> MNTNNIKKYAPQARNQFRDAVIQKLTTLGISADKKGNLQIADAELVGETMRYGQFDYPKSTLTRRDRLVKRAREQGFDVLVEHCAYTWFNRLCAIRYMEIHGYLDHGFHMLSHPDNPTGFEVLDHVPEVAEALLPEKKAQLVEMKLSGNQDEAIYRELLLAQCHALHRAMPFLFEAVDDEAELLLPDNLTRTDSILRGLVDGIPEEDWQEVEVIGWLYQFYISEKKDAVIGKVVKSEDIPAATQLFTPNWIVQYLVQNSVGRQWLQTYPDSPLKGKMDYYIEPAEQTPEVQAQLAAITPASIEPESIKVLDPACGSGHILIEVYNVLKNIYEERGYRARDIPQLILENNIFGLDIDDRAAQLSGFALLMMARQDDRRIFTRDVRLNIVSLQESLHLDIAKLWQQLNFHQQNQTGSMGDMFAENTALAHTDSAEYQLLMRTLKRFVNAKTLGSLIQVPQEEEAELKAFLEALYRMEQ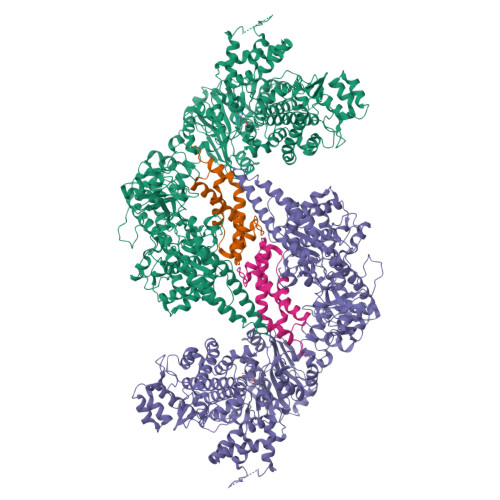EGDFQQKAAAKAFIPYIQQAWILAQRYDAVVANPPYMGGKGMNSELKEFAKNNFPDSKADLFAMFMQNAFSLLKENGFNAQVNMQSWMFLSSYEALRNWLLDNKTFITMAHLGARAFGQISGEVVQTTAWVIKNQHSERYQPVFFRLIDGREEVKKSDLLLRKNIFDKFTQHDFKNIPGMPIAYWIDLPSLLSFRHHKKLGEKIALKAGMSTGDNIKFQRYWYEVSIKKTLITNKESNTKIDIHNIKWFPCSSGGEYRKWYGNNEIVVNWENNGYEIRNFKFENGKTRSAVRNDEYYFREGITWSKISQGNFCVRYRPKGFVFDDTGRCGFSNNKNELLYAAGLMCTPVVNHYLSILAPTLSFTSGELASVPYPEIEDEIIELVTNAIEIAKNDWDSQEQSWDYVCSPLLEHNSTQLLRNIYKQKINTNIKLVETLLLIENTINNIFIDKLQLDKTIIKAVLQSEITLLCNPNYRYKNIQDHTDLTNKYYTDITIDILSYIIGCMMGRYSLDREGLVYAHEGNKGFAELVAEDAYKTFPADNDGILPLMDDEWFDDDVTSRVKEFVRTVWGEEHLQENLEFIAESLCLYAIKPKKGESALDTIRRYLSTQFWKDHMKMYKKRPIYWLFSSGKEKAFECLVYLHRYNDATLARMRTEYVVPLLARYQANIDRLNEQVDGASGGEATRLKRERDSLSKKFNELRSFDDRLRHYADMRISIDLDDGVKVNYGKFGDLLADVKAITGNAPEII;> MAMSNMTYNNVFDHAYEMLKENIRYDDIRDTDDLHDAIHMAADNAVPHYYADIFSVMASEGIDLEFEDSGLMPDTKDVIRILQARIYEQLTIDLWEDAEDLLNEYLEEVEEYEEDEE>[2x]GSHHVVPNEVVVQRLFQVKRRRVVRATEVPVSWESFNNGDCFILDLGNNIHQWC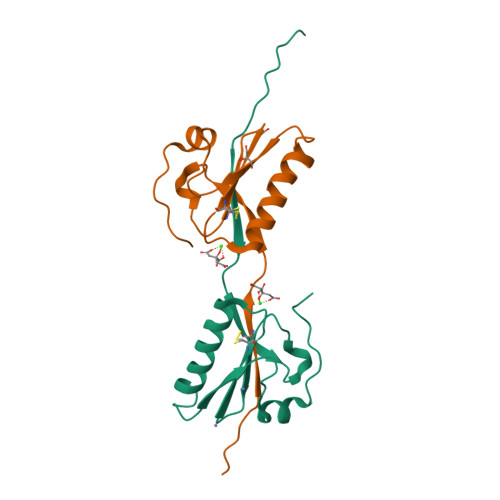GSNSNRYERLKATQVSKGIRDNERSGRARVHVSEEGTEPEAMLQVLGPKPALPAGTEDTAKEDAA> MLRSTLTSLNTFLTSSVATPPISVIRTGPKWWAHPERMVRQKLMYFTLGVDQLPLRRTAVIQRDLQRFHMCKPPP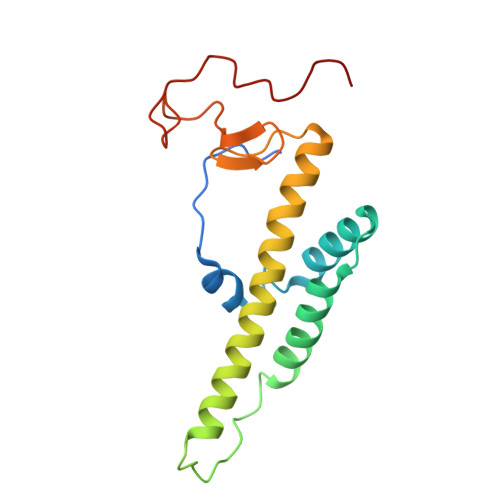RVGDSTGYKRSRAAQLNTWYRRIQYQEYHMQHLFTRHVWGLLRVYPGNTTKIQGKADDGYVGYDSVPFHRYNRAPLPFPARELYERRK>[2x]GPSFWLGNETLKVPLA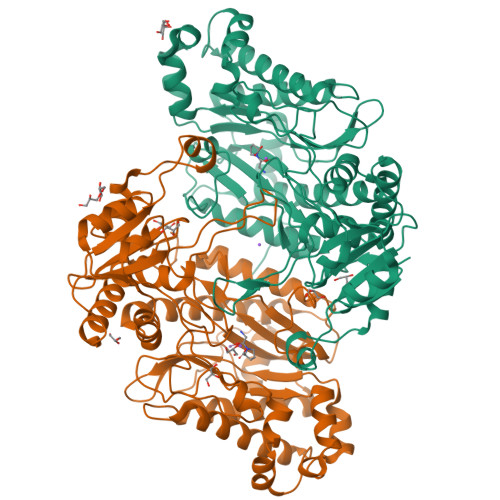LFALNRQRLCERLRKNPAVQAGSIVVLQGGEETQRYCTDTGVLFRQESFFHWAFGVTEPGCYGVIDVDTGKSTLFVPRLPASHATWMGKIHSKEHFKEKYAVDDVQYVDEIASVLTSQKPSVLLTLRGVNTDSGSVCREASFDGISKFEVNNTILHPEIVECRVFKTDMELEVLRYTNKISSEAHREVMKAVKVGMKEYELESLFEHYCYSRGGMRHSSYTCICGSGENSAVLHYGHAGAPNDRTIQNGDMCLFNMGGEYYCFASDITCSFPANGKFTADQKAVYEAVLRSSRAVMGAMKPGVWWPDMHRLADRIHLEELAHMGILSGSVDAMVQAHLGAVFMPHGLGHFLGIDVHDVGGYPEGVERIDEPGLRSLRTARHLQPGMVLTVEPGIYFIDHLLDEALADPARASFLNREVLQRFRGFGGVRIEEDVVVTDSGIELLTCVPRTVEEIEACMAGCDKAFTPFS> DMRPEIRIAQELRRXGD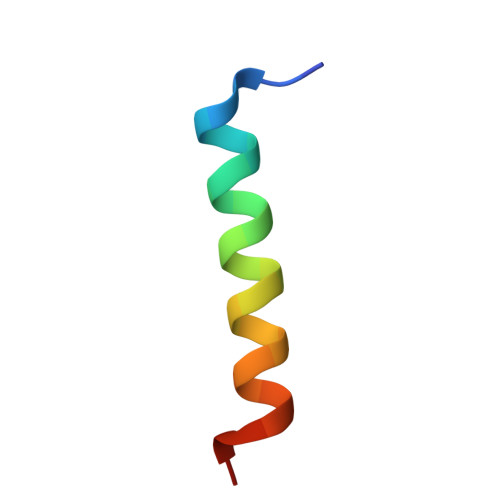EFNATYARR1-[[3,4-bis(fluoranyl)phenyl]methyl]-~{N}-[(1~{R})-2-[[(3~{E})-3-(1~{H}-imidazol-5-ylmethylidene)-2-oxidanylidene-1~{H}-indol-5-yl]amino]-2-oxidanylidene-1-phenyl-ethyl]-6-methyl-2-oxidanylidene-pyridine-3-carboxamide 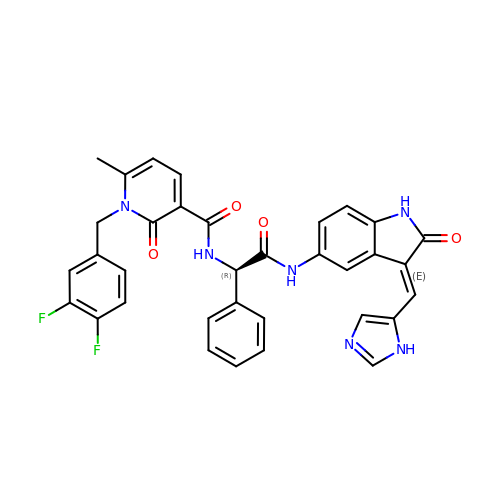| C34 H26 F2 N6 O4 | KHPDVVDNRUBARQ-WOZRVJTFSA-N>MPMTVITLKNVPQSLRGDLTRWMQEIATGVYVGNFNSRIREYLWRRVQETMGAGEASMCFAARNELGYDFLTENASRSVIDYDGLPLIFIPKEQSAVSDLPKGFSTAAKLHRAHIAGSGKKKEKPIRYVVIDIETDGKDAKRNHILEIGAIRCEDGKETHFTALISGDAVPPSITKLTGITATLLQKEGQEEKKVLTAFREFIGDDDLVGYHVSFDIEFLRQAFKKYGLGYLKNKTHDLLRIVKKEQLFQADYKLETSLQSYGIHKKVPHRALGDAELVKCLAKKLNKF[2x];>MAGPIIAGKSESSELPRVEDRATFIYIEHAKINRVD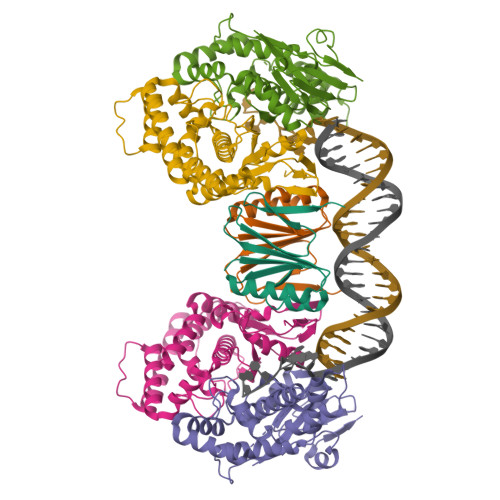SAVTVAEAKGVVRIPAAMIGVLLLGPGTDISHRAVELLGDTGTALVWVGEQGVRYYASGRALARSTRFLVKQAELVTNERSRLRVARRMYQMRFPTEDVSKLTMQQLRSHEGARVRRKYRELSKKYNVPWKKRVYNPDDFAGGDPINQALSAAHVALYGLVHSVVAALGLSPGLGFVHTGHDRSFIYDVADLYKAEITVPIAFAVAAEAEEGQDIGQLARLRTRDAFVDGKILKRMVKDLQTLLEIPEEGQIEAEPLSLWDDKEKLVPYGVNYSEVTSCP[4x]> GSHMGLKIQYYSRKPHDSAGIDFSFRMFNTGNEAIDLKDVKVRYYFKEDVSIDEMNWAVYFYSLGSEKDVQCRFYELPGKKEANKYLEITFK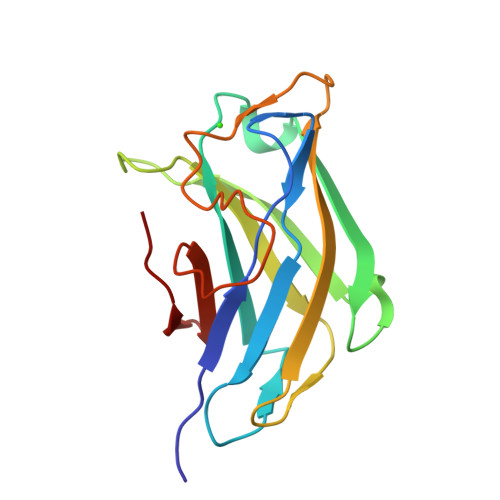SGTLSPNDVMYITGEFYKNDWTKFEQRDDYSYNPADSYSDWKRMTAYISNKLVWGIEP> MRLSYEALEWRTPIENSTEPVSLPPPPPFFGQERAREALELAIRGGFHAYLVGPPSLGKHEALLAYLSTQSVETPPDLLYVPLSERKVAVLTLPSGQEIHLAEAVEGLLLEVNRLDELFRQGSFLREKTQLEARFKEAREQQLEALRREAQEAGFALSTNGERLELTGPGPVPAELSARLEEVTLGSLAASAELEVALRRLRRDWALHYLNNRFEPLFQRFPQARAYLEALRARLARYAETGEPLDPAQWRPNLLTSSSSGTPPPIVYEPYATAPRLFGRLDYLVDRGVWSTNVSLIRPGAVHRAQGGYLILDALSLKREGTWEAFKRALRNGQVEPVTEPQAPAGLEVEPFPIQMQVILVGTPEAFEGLEEDPAFSELFRIRAEFSPTLPASPENCTALGGWLLAQGFQLTQGGLTRLYDEARRMAEQRDRMDARLVEIRALAEEAAVLGGGLLTAE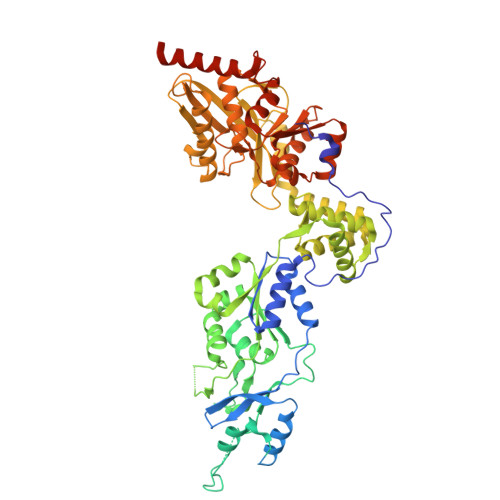SVEQAIAAREHRSFLSEEEFLRAVQEGVIRLRTTGRAVGEVNSLVVVEAAPYWGRPARLTARAAPGRDHLISIDREAGLGGQIFHKAVLTLAGYLRSRYIEHGSLPVTISLAFEQNYVSIEGASAGLAELVAALSAIGNLPLRQDLAVTGAVDQTGKVLAVGAINAKVEGFFRVCKALGLSGTQGVILPEANLANLTLRAEVLEAVRAGQFHIYAVETAEQALEILAGARMEGFRGLQEKIRAGLEAFARLEEGHDKEDREKLAAALEHHHHHH OXIDIZED COENZYME A | C21 H36 N7 O17 P3 S | 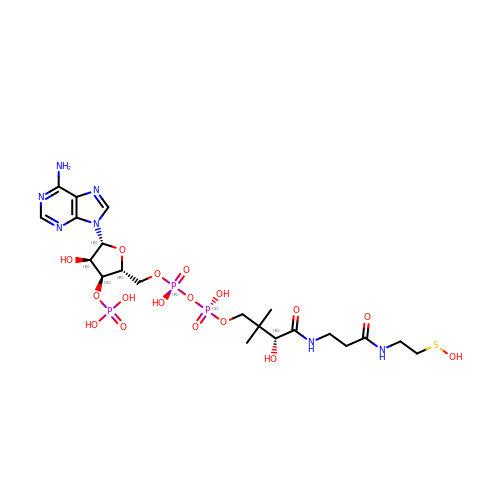HWMGJMKHOJKGLQ-IBOSZNHHSA-N N-(3-OXOPROPYL)GLYCINE | 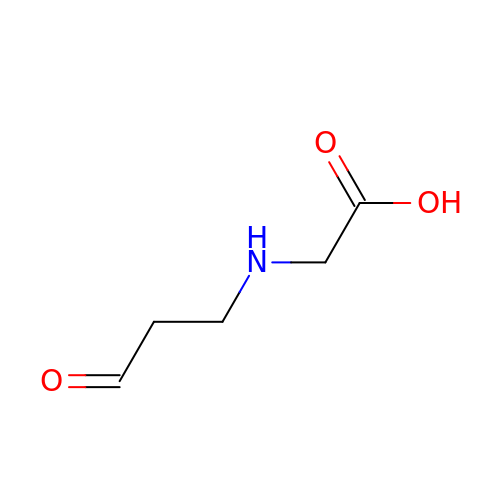C5 H9 N O3 | KCNYJRBIWGISEE-UHFFFAOYSA-N> NLRARLAKTSNRDDPIRPPLKVARSPRPGQCQDVVQDVPNVDVQMLELYDRMSFKDIDGGVWKQGWNIKYDPLKYNAHHKLKVFVVPHSHNDPGWIQTFEEYYQHDTKHILSNALRHLHDNPEMKFIWAEISYFARFYHDLGENKKLQMKSIVKNGQLEFVTGGWVMPDEANSHWRNVLLQLTEGQTWLKQFMNVTPTASWAIDPFGHSPTMPYILQKSGFKNMLIQRTHYSVKKELAQQRQLEFLWRQIWDNKGDTALFTHMMPFYSYDIPHTCGPDPKVCCQFDFKRMGSFGLSCPWKVPPRTISDQNVAARSDLLVDQWKKKAELYRTNVLLIPLGDDFRFKQNTEWDVQRVNYERLFEHINSQAHFNVQAQFGTLQEYFDAVHQAERAGQAEFPTLSGDFFTYADRSDNYWSGYYTSRPYHKRMDRVLMHYVRAAEMLSAWHSWDGMARIEERLEQARRELSLFQHHDGITGTAKTHVVVDYEQRMQEALKACQMVMQQSVYRLLTKPSIYSPDFSFSYFTLDDSRWPGSGVEDSRTTIILGEDILPSKHVVMHNTLPHWREQLVDFYVSSPFVSVTDLANNPVEAQVSPVWSWHHDTLTKTIHPQGSTTKYRIIFKARVPPMGLATYVLTISDSKPEHTSYASNLLLRKNPTSLPLGQYPEDVKFGDPREISLRVGNGPTLAFSEQGLLKSIQLTQDSPHVPVHFKFLKYGVRSHGDRSGAYLFLPNGPASPVELGQPVVLVTKGKLESSVSVGLPSVVHQTIMRGGAPEIRNLVDIGSLDNTEIVMRLETHIDSGDIFYTDLNGLQFIKRRRLDKLPLQANYYPIPSGMFIEDANTRLTLLTGQPLGGSSLASGELEIMQDRRLASDDERGLGQGVLDNKPVLHIYRLVLEKVNNCVRPSKLHPAGYLTSAAHKASQSLLDPLDKFIFAENEWIGAQGQFGGDHPSAREDLDVSVMRRLTKSSAKTQRVGYVLHRTNLMQCGTPEEHTQKL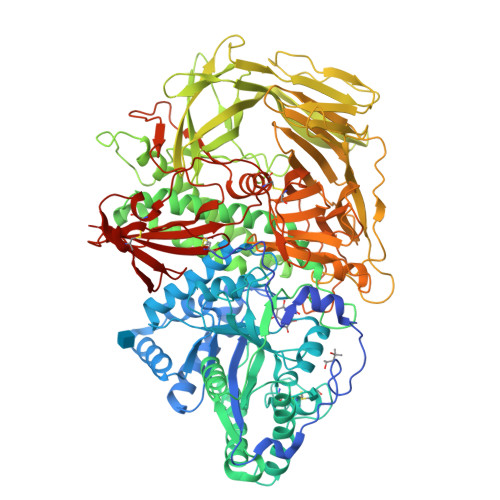DVCHLLPNVARCERTTLTFLQNLEHLDGMVAPEVCPMETAAYVSSHSS> MHHHHHHSSGRENLYFQGLSDRYQRVKKLGSGAYGEVLLCKDKLTGAERAIKIIKKSSVTTTSNSGALLDEVAVLKQLDHPNIMKLYEFFEDKRNYYLVMEVYRGGELFDEIILRQKFSEVDAAVIMKQVLSGTTYLHKHNIVHRDLKPENLLLESKSRDALIKIVDFGLSAHFEVGGKMKERLGTAYYIAPEVLRKKYDEKCDVWSCGVILYILLCGYPPFGGQT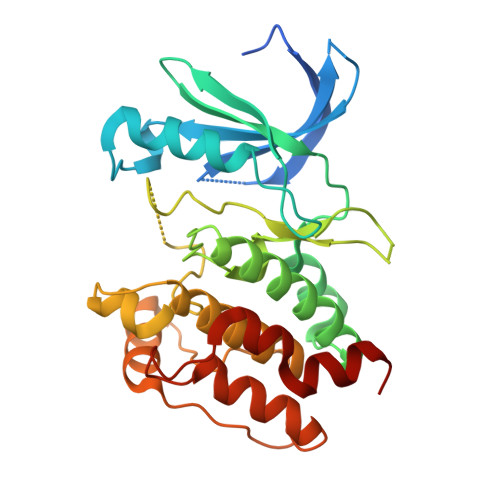DQEILKRVEKGKFSFDPPDWTQVSDEAKQLVKLMLTYEPSKRISAEEALNHPWIVKFCSQK>[2x]GTRSESTEGHSKDLLYKYKLYGDIDEYAYYFLDIDIGTPEQRISLILDTGSSSLSFPCAGCKNCGVHMENPFNLNNSKTSSILYCENEECPFKLNCVKGKCEYMQSYCEGSQISGF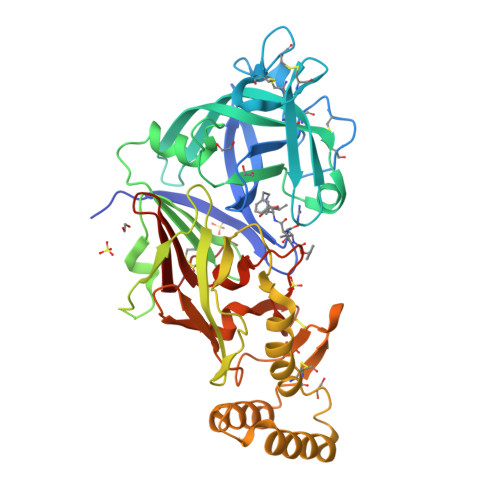YFSDVVSVVSYNNERVTFRKLMGCHMHEESLFLYQQATGVLGMSLSKPQGIPTFVNLLFDNAPQLKQVFTICISENGGELIAGGYDPAYIVRRGGSKSVSGQGSGPVSESLSESGEDPQVALREAEKVVWENVTRKYYYYIKVRGLDMFGTNMMSSSKGLEMLVDSGSTFTHIPEDLYNKLNYFFDILCIQDMNNAYDVNKRLKMTNESFNNPLVQFDDFRKSLKSIIAKENMCVKIVDGVQCWKYLEGLPDLFVTLSNNYKMKWQPHSYLYKKESFWCKGIEKQVNNKPILGLTFFKNRQVIFDIQKNRIGFVDANCPSHPTHTRPR> FVGGVV;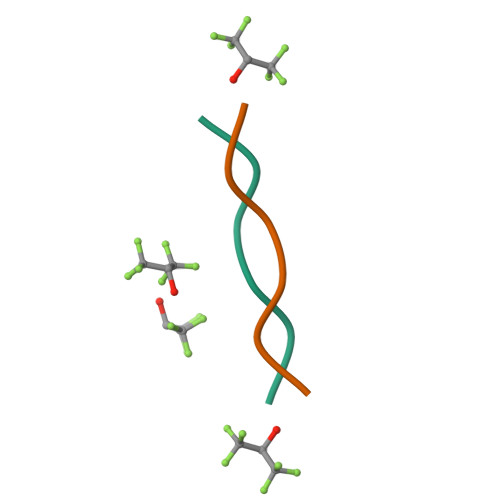> MVGGVV>[4x]GMKKKNVIVFGGGTGLSVLLRGLKTFPVSITAIVTVADDGGSSGRLRKELDIPPPGDVRNVLVALSEVEPLLEQLFQHRFENGNGLSGHSLGNLLLAGMTSITGDFARGISEMSKVLNVRGKVLPASNRSIILHGEMEDGTIVTGESSIPKAGKKIKRVFLTPKDTKPLREGLEAIRKADVIVIGPGSLYTSVLPNLLVPGICEAIKQSTARKVYICNVMTQNGETDGYTASDHLQAIMD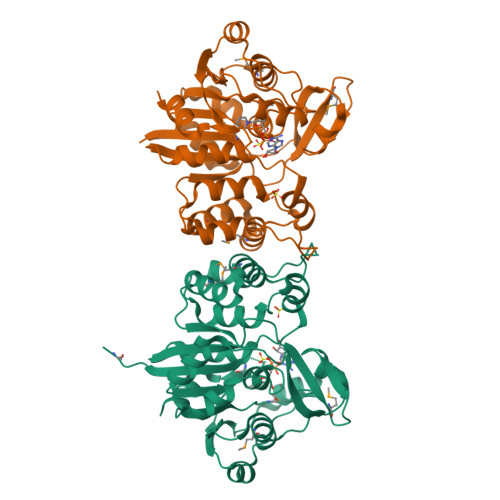HCGVGIVDDILVHGEPISDTVKAKYAKEKAEPVIVDEHKLKALGVGTISDYFVLEQDDVLRHNASKVSEAILEGKPRTSSSIQ> MAIAFEHVTYTYQAGTPMAHTALTDVSLTVPDRGYLAIIGHTGSGKSTLIQQLNALLKPTSGTIKIDEFTITPETTNAALKPLRQHVGMVFQFPENQLFEETVRQDIAFG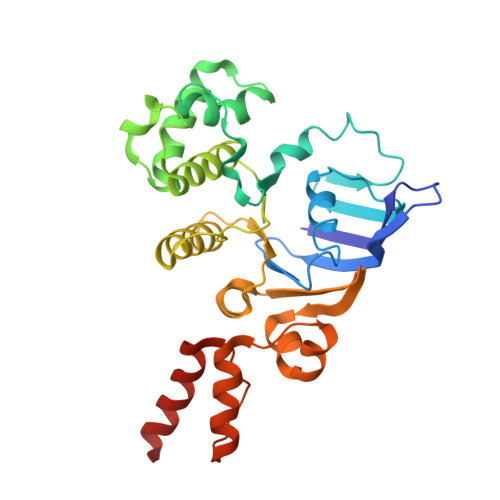PKNFGMADADALALADEMLTTVGLDQSYAERSPFELSGGQMRRVAIAGVLAMQPKVLVLDEPTAGLDPQGRQEMMRLFARLHQEQGLTIVLVTHQMEDVAQYAEQVAVMHEGRLMKFGTPADVFSNREWLQDHQLDVPQAAQFARRLRDRGLTFPKQPLTADQLADYLAQQWAQRGADHV> EVSAEEIKKHEEKWNKYYGVNAFNLPKELFSKVDEKDRQKYPYNTIGNVFVKGQTSATGVLIGKNTVLTNRHIAKFANGDPSKVSFRPSINTDDNGNTETPYGEYEVKEILQEPFGAGVDLALIRLKPDQNGVSLGDKISPAKIGTSNDLKDGDKL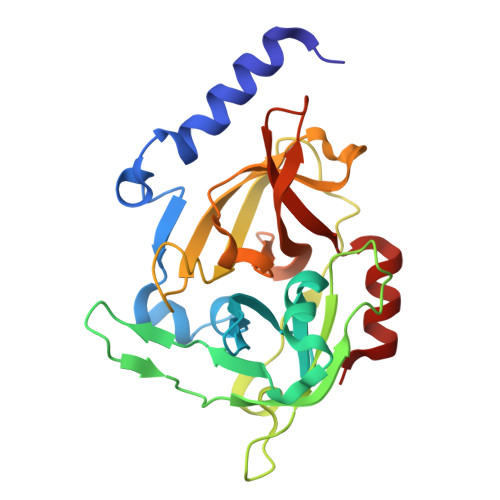ELIGYPFDHKVNQMHRSEIELTTLSRGLRYYGFTVPGNSGSGIFNSNGELVGIHSSKVSHLDREHQINYGVGIGNYVKRIINEKNE> HHHHHHMSPIEPAASAIFGPRLGLARRYAEALAGPGVERGLVGPREVGRLWDRHLLNCAVIGELLERGDRVVDIGSGAGLPGVPL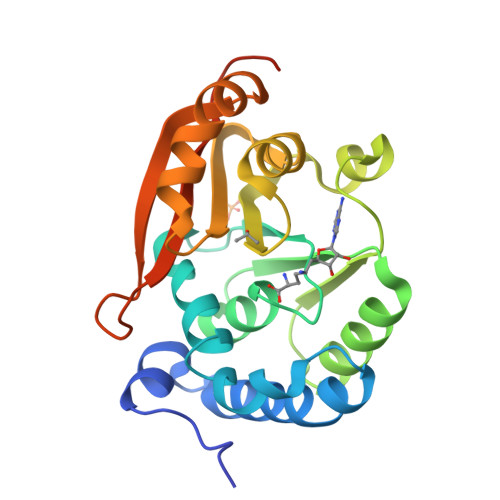AIARPDLQVVLLEPLLRRTEFLREMVTDLGVAVEIVRGRAEESWVQDQLGGSDAAVSRAVAALDKLTKWSMPLIRPNGRMLAIKGERAHDEVREHRRVMIASGAVDVRVVTCGANYLRPPATVVFARRGKQIARGSARMASGGTA> GSHMRNVAAEQQLRELESTFDGRLGFVALDTATGARIAHRADERFPFCSTFKTMLSAAVLARSAGDAALLQRRIPYAKRDLVRYSPITEKHVGAGMTVAELCAATLQYSDNTAANLLIALLGGPQAVTAYARSIGDATFRLDRRETELNTAIPGDERDTTTPA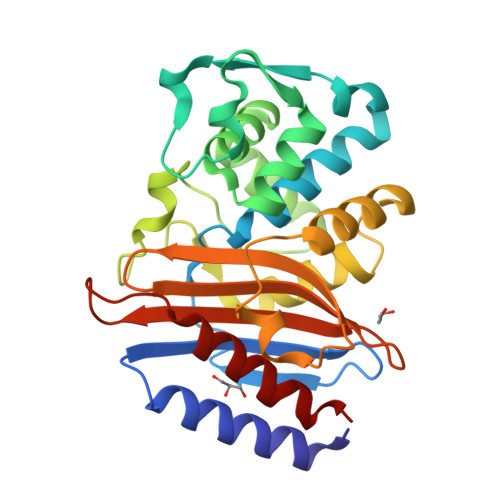AMAASVRRLLVGDALGTAQRAQLNAWMLGNKTGDARIRAGVPAGWRVADKTGTGDYGTGNDIGVAYPPDRAPIVFVVYTTMRSRNAQARDDVIASAARIAARAFV Tipα, therefore, is an important pathogenic effector of H. pylori that promotes host inflammation and tumor progression. Tipα is secreted as homodimer by H. pylori independent of the type IV secretion system. The active form of Tipα can bind the gastric epithelial cells and subsequently be translocated into the cytoplasm.

Here we report the crystal structure of the N-terminal-truncated Tipα starting from the residue Cys25 (TipαN25) that retains both inter-molecular disulfide bridges. Our TipαN25 is always dimer independent of pH values or protein concentrations under non-reductive conditions. In the crystal structure, TipαN25 adopts an intrinsic dimeric organization as the active unit, which features two flexible disulfide bonds at the N-terminus linking two monomers of the unit to form a tweezer-like configuration. A homodimer, linked by inter-subunit disulfide bonds at the N-terminus, is present in an asymmetric unit. Two subunits of a TipαN25 homodimer related by a local twofold axis are arranged in an anti-parallelly way to form a unique shoulder-to-shoulder dimeric mode. The N-terminal loops (25–33), where the two inter-chain disulfide bonds are located are structurally flexible and not visible in the experimental electron density map, implying their nature of intrinsic flexibility. Tethered by flexible disulfide bonds at the N-terminus, two subunits of TipαN25 are assembled in an almost anti-parallel shoulder-to-shoulder mode with the dimer interface mainly mediated through β sheets. The whole structure of TipαN25 homodimer resembles the shape of a pair of tongs, with the disulfide bridges as pivot and a pair of anti-parallel β sheets as jaws of the tongs to clip targets for its functional performances. The dimer interface buries a contact area of 4813.3Å2, reaching 30% of the total accessible surface area, which is primarily contributed by β sheets.

>[2x]CTCPNTSQRNSFLQDVPYWMLQNRSEYITQGVDSSHIVDGKKTEEIEKIATKRATIRVAQNIVHKLKEAYLSKTNRIKQKITNEMFIQMTQPIYDSLMNVDRLGIYINPNNEEVFALVRARGFDKDALSEGLHKMSLDNQAVSILVAKVEEIFKDSVNYGDVKVPIAM>[2x]TQAHSENKCSGASQKLPRKMVAIDCEMVGTGPKGHVSSLARCSIVNYNGDVLYDEYILPPCHIVDYRTRWS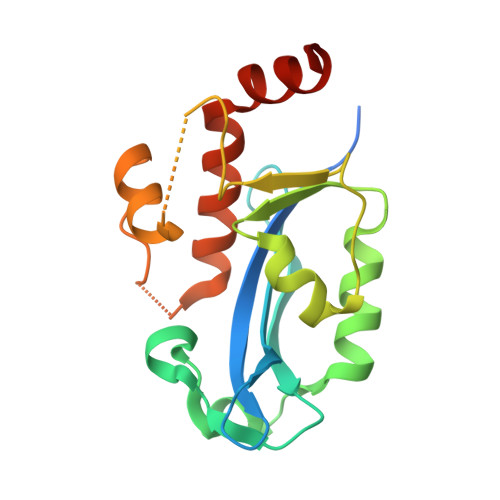GIRKQHMVNATPFKIARGQILKILTGKIVVGHAIHNDFKALQYFHPKSLTRDTSHIPPLNRKADCPENATMSLKHLTKKLLNRDIQVGKSGHSSVEAAQATMELYKLVEVEWEEHLARNPPTD>APEEERIKYVITVVEQIAKDAHRNGQEELAKLAERTAEEAKKATERGEEETLRIVYVIVVVLQIALEAHRNGQEELAKLALRTAEEAIKATERGEEETLRIVYVIVVVLQIALEAHRNGQEELAKLALRTAEEAIKATERGEEETLRIVYVIVVVLQIALEAHRNGQEELAKLALRTAEEAIKATERGEEETLRIVYVIVVVLQIALEAHRNGQEELAKLALRTAEEAIKATERGEEETERIVYDIVVVLQEALEAHRNGEEERAKKALDEARRRIEATERGE[2x];> P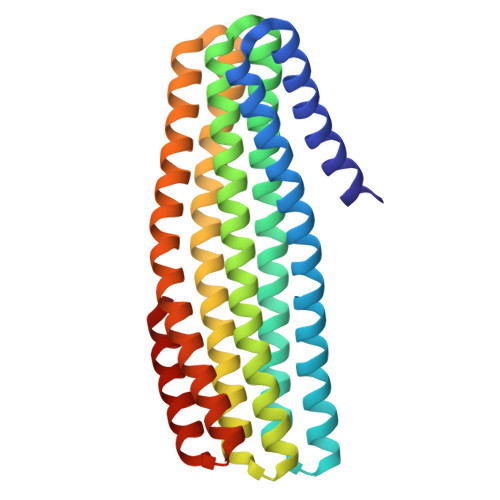LPPLPPLPPLPPLPPLP> MFGSGNVLPVKIQPPLLRPLAYRVLSRKYGLSIKSDGLSALAEFVGTNIGANWRQGPATIKFLEQFAAVWKQQERGLFIDQSGVKEVIQEMKEREKVEWSHEHPIQHEENILGRTDDDENNSDDEMPIAADSSLQNVSLSSPMRQPTERDEYKQPFKPESSKALDWRDYFKVINASQQQRFSYNPHKMQFIFVPNKKQNGLGGIAGFLPDIEDKVQMFLTRYYLTNDRVMRNENFQNSDMFNPLSSMVSLQNELSNTNRQQQSSSMSITPIKNLLGRDAQNFLLLGLLNKNFKGNWSLEDPSGSVEIDISQTIPTQGHYYVPGCMVLVEGIYYSVGNKFHVTSMTLPPGERREITLETI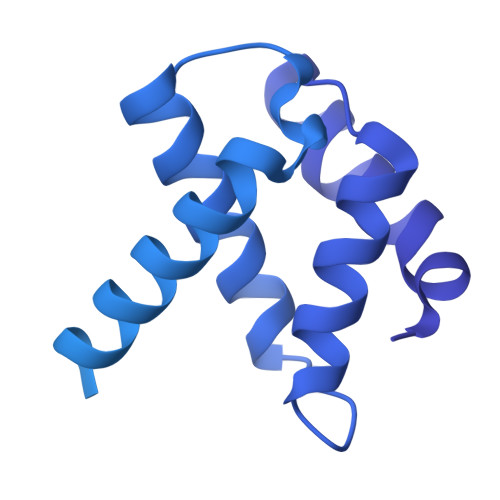GNLDLLGIHGISNNNFIARLDKDLKIRLHLLEKELTDHKFVILGANLFLDDLKIMTALSKILQKLNDDPPTLLIWQGSFTSVPVFASMSSRNISSSTQFKNNFDALATLLSRFDNLTENTTMIFIPGPNDLWGSMVSLGASGTLPQDPIPSAFTKKINKVCKNVVWSSNPTRIAYLSQEIVIFRDDLSGRFKRHRLEFPFNESEDVYTENDNMMSKDTDIVPIDELVKEPDQLPQKVQETRKLVKTILDQGHLSPFLDSLRPISWDLDHTLTLCPIPSTMVLCDTTSAQFDLTYNGCKVINPGSFIHNRRARYMEYVPSSKKTIQEEIYI> ASNLKIVRMDRTAGCVTGGEEIYLLCDKVQKDDIQIRFYEEEE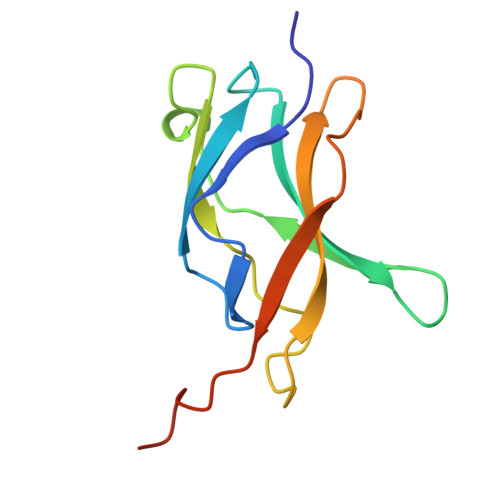NGGVWEGFGDFSPTDVHRQFAIVFKTPKYKDVNITKPASVFVQLRRKSDLETSEPKPFLYYPEIKDKEEVQRKRQK> MASWSHPQFEKSGGGGGENLYFQGAVLALERHFEKVEEILKKYGYKRENLIKILLEIQEIYRYLPEDVINYVSTAMGIPPAKIYGVATFYAQ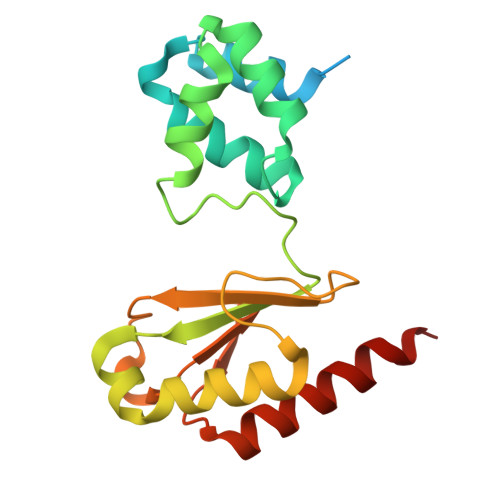FSLKPKGKYTIMVCDGTACHMAGSPEVLKAIEEETGLTPGNVTEDLMFSLDQVGCLGACALAPVMVINGEVYGNLTADKVKEILRKIKEKERESANV> QAVTAFLGERVTLTSYWRRVSLGPEIEVSWFKLGPGEEQVLIGRMHHDVIFIEWPFRGFFDIHRSANTFFLVVTAANISHDGNYLCRMKLGETEVTKQEHLSVVKPLTLSVHSERSQFPDFSVLTVTCTVNAFPHPHVQWLMPEGVEPAPTAANGGVMKEKDGSLSVAVDLSLPKPWHLPVTCVGKNDK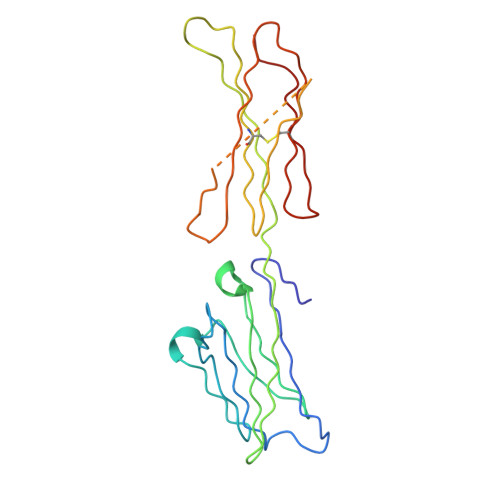EEAHGVYVSGYLSQ In M. tuberculosis, the cell wall contains high levels of 3 → 3 (meso-Dap–meso-Dap) cross-links (approx. 80% at stationary phase), which are formed by the l,d-transpeptidases (Ldts) (ESI†).6 Evidence has emerged that LdtMt2, in particular, plays an important role in the virulence of M. tuberculosis, as disruption of the ldtMt2 gene results in altered morphology and inhibition of colony growth. Mechanistically, the Ldts differ from the PBPs through their use of a nucleophilic cysteine rather than serine during catalysis. Several β-lactam antibiotics, in particular carbapenems, have been shown to inhibit the activity of LdtMt2 and to have anti-TB activity. Such LdtMt2 inhibition involves covalent modification of the nucleophilic cysteine (Cys354), which reacts with β-lactam antibiotics to give (a) stable acyl–enzyme complex(es). Consistent with previous reports, the structure of LdtMt2 consists of two N-terminal immunoglobulin fold-related domains and a C-terminal catalytic domain.

Structural studies on LdtMt2 with potent inhibitor ebselen reveal opening of the benzisoselenazolone ring by a nucleophilic cysteine, forming a complex involving extensive hydrophobic interactions with a substrate-binding loop. LdtMt2 crystals were soaked with ebselen, and the structure of the complex was solved by molecular replacement (ESI†). In both protein chains in the ASU, electron density consistent with the presence of a single ebselen-derived adduct was observed extending from Cys354. While a single ebselen conformation was refined in chain B (conformation II), two different conformations were refined in chain A (conformations I and II). The ratio of conformations I and II in chain A appeared to depend on the length of time that LdtMt2 crystals were soaked with ebselen, with the conformation corresponding to that observed in chain B (i.e., conformation II) predominating at longer time points (data not shown). Extensive hydrophobic interactions are apparent between both aromatic rings of ebselen and the LdtMt2 active site in conformations I and II. In addition to Val333, Phe334 and His352, residues from the mobile active-site loop (a two-stranded β-sheet encompassing residues 300–323) including Met303, Tyr308, Tyr318, and Thr320, contribute to the hydrophobic pocket around Cys354. Apparent pi-stacking between the phenol ring of Tyr318 and the ebselen-derived phenyl ring proximal to Cys354 (ring A in Fig. 2A) is present in conformations I and II; this interaction has also been observed in the complex derived from LdtMt2 and 5,5′-dithiobis-(2-nitrobenzoic acid). The position of the ebselen-derived phenyl ring distal to Cys354 (ring B) depends on the conformation of ebselen; in conformation I, ring B appears to pi-stack with His352, while in conformation II, it interacts primarily with Val333.

>SMDLLVPKLTASVTDGAVGVTVDAPVSVTAADGVLAAVTMVNDNGRPVAGRLSPDGLRWSTTEQLGYNRRYTLNATALGLGGAATRQLTFQTSSPAHLTMPYVMPGDGEVVGVGEPVAIRFDENIADRGAAEKAIKITTNPPVEGAFYWLNNREVRWRPEHFWKPGTAVDVAVNTYGVDLGEGMFGEDNVQTHFTIGDEVIATADDNTKILTVRVNGEVVKSMPTSMGKDSTPTANGIYIVGSRYKHIIMDSSTYGVPVNSPNGYRTDVDWATQISYSGVFVHSAPWSVGAQGHTNTSHGCLNVSPSNAQWFYDHVKRGDIVEVVNTVGGTLPGIDGLGDWNIPWDQWRAGNAKA[2x]> GPGSSHRHSAIIVPSYRPTP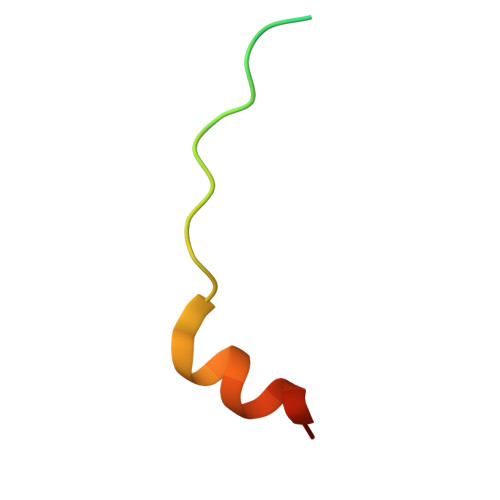DYETVMRQMKRG1-[(4-bromanyl-2-fluoranyl-phenyl)methyl]-4-chloranyl-pyrazolo[3,4-d]pyrimidin-6-amine 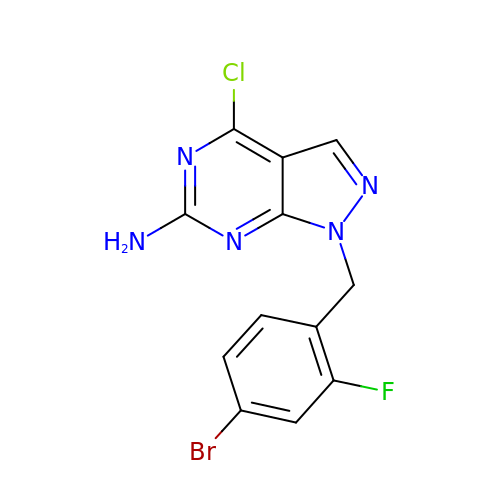| C12 H8 Br Cl F N5 | UKBISIPKUKNJKU-UHFFFAOYSA-N> SDEFDALRIKWATLLTGGPALDPADSDIAARTDKLAQDAN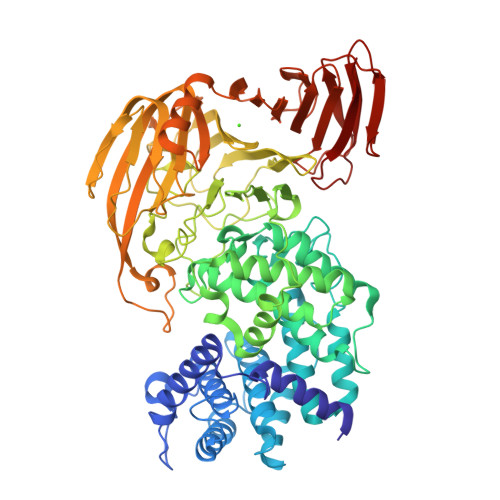DYWEDMDLSSSRTYIWYALRGNGTSDNVNAVYERLRTMALAATTVGSSLYGNADLKEDILDALDWLYVNSYNSTRSRSAYNWWHWQLGIPMSLNDTAVLLYDDISAARMATYMDTIDYFTPSIGLTGANRAWQAIVVGVRAVIVKDAVKLAAARNGLSGTGIFPYATGGDGFYADGSFVQHTTFAYTGGYGSSVLETTANLMYLLSGSTWSVSDPNQSNVWQWIYEAYRPLLYKGAMMDMVRGREISRSYAQDHAVGHGIVASIVRLAQFAPAPHAAAFKQIAKRVIQEDTFSSFYGDVSTDTIRLAKAIVDDPSIAPAAAPNLYKQYAAMDRAVLQRPGFALGLALYSTRISSYESINSENGRGWYTGAGATYLYNQDLAQYSEDYWPTVDAYRIPGTTVASGTPIASGTGTSSWTGGVSLAGQYGASGMDLSYGAYNLSARKSWFMFDDEIVALGSGISSTAGIPIETVVDNRKLNGAGDNAWTANGAALSTGLGVAQTLTGVNWVHLAGNTADGSDIGYYFPGGATLQTKREARTGTWKQINNRPATPSTAVTRNYETMWIDHGTNPSGASYGYVLLPNKTSAQVGAYAADPAIEIVVNTSGVQSVKEKTLGLVGANFWTDTTQTADLITSNKKASVMTREIADERLEASVSDPTQANNGTIAIELARSAEGYSADPGITVTQLAPTIKFTVNVNGAKGKSFHASFQLG>[2x]MGPYRRLWFTLIAVLAVTFALLGFYGGEVYRQAP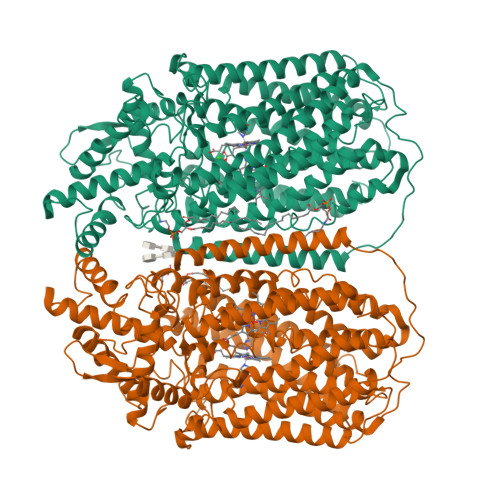PIPEEVASADGTRLFGRDDILDGQTAWQSIGGMQLGSIWGHGAYQAPDWTADWLHRELMAWLDLAARDAHGRDYGQLDAPAQAALREQLKAEYRANRADAAGGKLTLSPRRAQAVAQTEAYYDQLFSDAPALHRSRENYAMKENTLPDANRRRQMTHFFFWTAWAAGTEREGTSVTYTNNWPHEPLIGNHPSSENVMWSIISVVVLLAGIGLLIWAWAFLRGKEEDEPPAPARDPLTTFALTPSQRALGKYLFLVVALFGFQVLLGGFTAHYTVEGQKFYGIDLSQWFPYSLVRTWHIQSALFWIATGFLAAGLFLAPLINGGRDPKYQKAGVDILFWALVLVVVGSFAGNYLAIAQIMPPDLNFWLGHQGYEYVDLGRLWQIGKFAGICFWLVLMLRGIVPALRTPGGDKNLLALLTASVGAIGLFYGAGFFYGERTHLTVMEYWRWWIVHLWVEGFFEAFATTALAFIFSTLGLVSRRMATTASLASASLFMLGGIPGTFHHLYFAGTTTPVMAVGASFSALEVVPLIVLGHEAWENWRLKTRAPWMENLKWPLMCFVAVAFWNMLGAGVFGFMINPPVSLYYIQGLNTTPVHAHAALFGVYGFLALGFTLLVLRYIRPQYALSPGLMKLAFWGLNLGLALMIFTSLLPIGLIQFHASVSEGMWYARSEAFMQQDILKTLRWGRTFGDVVFLLGALAMVVQVILGLLSGK3-({4-[(5-chloro-1,3-benzodioxol-4-yl)amino]pyrimidin-2-yl}amino)benzenesulfonamide 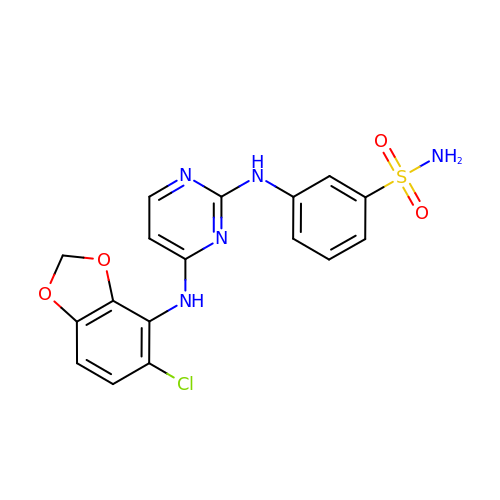| C17 H14 Cl N5 O4 S | TZHCXOMEOHEZDX-UHFFFAOYSA-N>[2x]MDRPAVSGPMDLPIMHDSDRYELVKDIGSGNFGVARLMRDKQSNELVAVKYIERGEKIDENVKREIINHRSLRH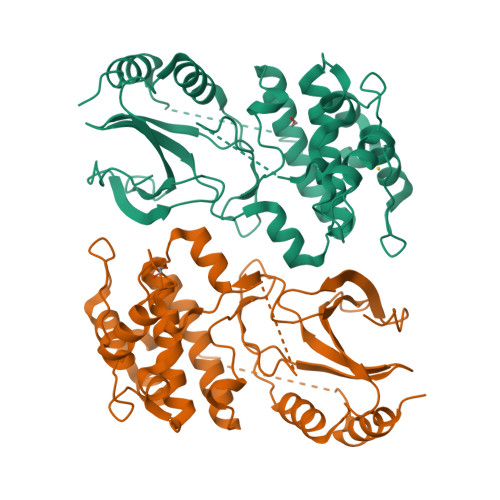PNIVRFKEVILTPTHLAIVMEYASGGELFERICNAGRFSEDEARFFFQQLISGVSYCHAMQVCHRDLKLENTLLDGSPAPRLKICAFGYSKSSVLHSQPKDTVGTPAYIAPEVLLKKEYDGKVADVWSCGVTLYVMLVGAYPFEDPEEPKNFRKTIHRILNVQYAIPDYVHISPECRHLISRIFVADPAKRISIPEIRNHEWFLKNLPADLMNDNTMTTQFDESDQPGQSIEEIMQIIAEATVPPAGTQNLNHYLTGSLDIDDDMEEDLESDLDDLDIDSSGEIVYAM> MTQAKAKHADVPVNLYRPNAPFIGKVISN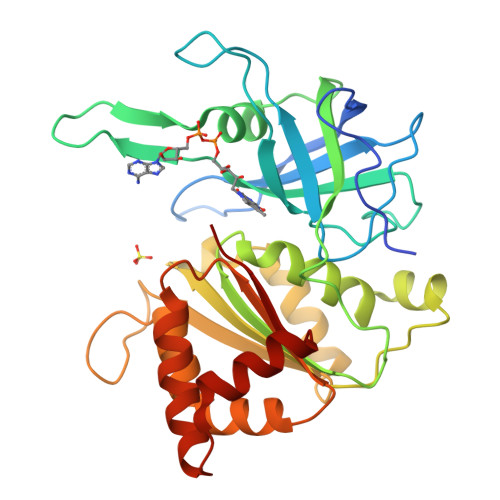EPLVKEGGIGIVQHIKFDLTGGNLKYIEGQSIGIIPPGVDKNGKPEKLRLYSIASTRHGDDVDDKTISLCVRQLEYKHPESGETVYGVCSTYLTHIEPGSEVKITGPVGKEMLLPDDPEANVIMLATGTGIAPMRTYLWRMFKDAERAANPEYQFKGFSWLVFGVPTTPNILYKEELEEIQQKYPDNFRLTYAISREQKNPQGGRMYIQDRVAEHADQLWQLIKNQKTHTYICGLRGMEEGIDAALSAAAAKEGVTWSDYQKDLKKAGRWHVETS>[2x]NVHSNYTFIIAGGGISGLTLADRLTEDPRVTVLVIEAGPLDRGEDGILVPGAFSPWLYFWPGLVSTPQAGLNNRTVDVITAQVVGGGSTINAMVYLRGDKDDYDSWGALGNPGWSWNSMLPYFIKSETFTPPSPELAAAGNITWDGSIRGRSGPVNYSYPNYFFPGSENWWNAANEVGLPPVKDPMAGSKQGVFWIPSAIDARTMTRSHARRNHYDRVSSRPNYHILPSHLVSKILFRGKQAIGVSYIPTSGGNTTTNVYASKEITLAAGGLGTPKILQLSGIGPRKLLNELGIPVISDLPGVGQNLQDQPTLTIPYTFTNNVFPNTDSLTTNATYNAEQRALYDSSKQGAYTIVNSLSTNIGVMSLQRAAPKSYRQIIAAARARSASLSLPPGTDPAVIRGYQAQRNAIL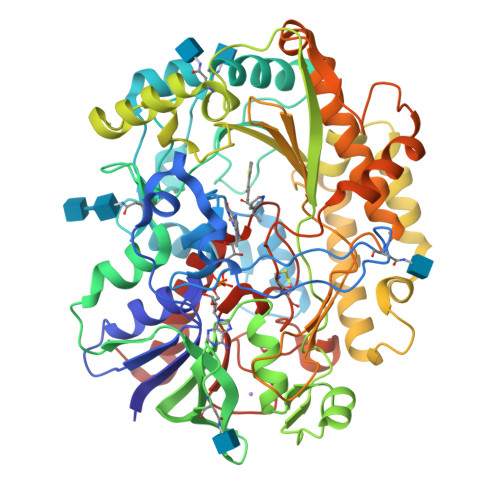KQFENPNVGVGTVHWGTGSSALVYHLKPLSRGTVNIRSTNPLDAPEIDYRTGTDPIDAQVYTSLFRKNREIFNAPSMRVLGPSEAAPFGANLTTDEEIYAVMRELINPSNAHQCCTAAMMPKDMGGVVSSEQKVYGVQGLRVADISFWPFQLSGSPMATAYAGAERLADVIKKEHRLAGAPKSL> DDPIRPPLKVARSPRPGQCQDVVQDVPNVDVQMLELYDRMSFKDIDGGVWKQGWNIKYDPLKYNAHHKLKVFVVPHSHNDPGWIQTFEEYYQHDTKHILSNALRHLHDNPEMKFIWAEISYFARFYHDLGENKKLQMKSIVKNGQLEFVTGGWVMPDEANSHWRNVLLQLTEGQTWLKQFMNVTPTASWAIDPFGHSPTMPYILQKSGFKNMLIQRTHYSVKKELAQQRQLEFLWRQIWDNKGDTALFTHMMPFYSYDIPHTCGPDPKVCCQFDFKRMGSFGLSCPWKVPPRTISDQNVAARSDLLVDQWKKKAELYRTNVLLIPLGDDFRFKQNTEWDVQRVNYERLFEHINSQAHFNVQAQFGTLQEYFDAVHQAERAGQAEFPTLSGDFFTYADRSDNYWSGYYTSRPYHKRMDRVLMHYVRAAEMLSAWHSWDGMARIEERLEQARRELSLFQHHDGITGTAKTHVVVDYEQRMQEALKACQMVMQQSVYRLLTKPSIYSPDFSFSYFTLDDSRWPGSGVEDSRTTIILGEDILPSKHVVMHNTLPHWREQLVDFYVSSPFVSVTDLANNPVEAQVSPVWSWHHDTLTKTIHPQGSTTKYRIIFKARVPPMGLATYVLTISDSKPEHTSYASNLLLRKNPTSLPLGQYPEDVKFGDPREISLRVGNGPTLAFSEQGLLKSIQLTQDSPHVPVHFKFLKYGVRSHGDRSGAYLFLPNGPASPVELGQPVVLVTKGKLESSVSVGLPSVVHQTIMRGGAPEIRNLVDIGSLDNTEIVMRLETHIDSGDIFYTDLNGLQFIKRRRLDKLPLQANYYPIPSGMFIEDANTRLTLLTGQPLGGSSLASG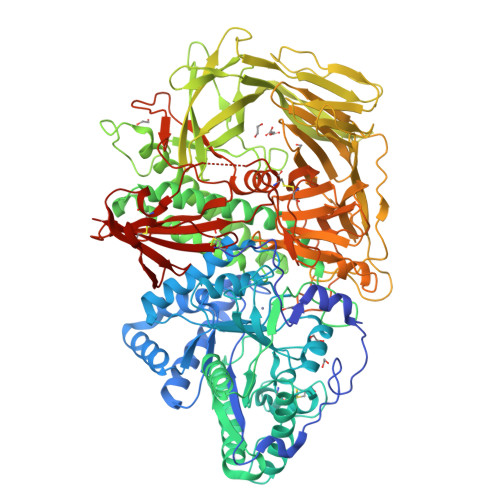ELEIMQDRRLASDDERGLGQGVLDNKPVLHIYRLVLEKVNNCVRPSELHPAGYLTSAAHKASQSLLDPLDKFIFAENEWIGAQGQFGGDHPSAREDLDVSVMRRLTKSSAKTQRVGYVLHRTNLMQCGTPEEHTQKLDVCHLLPNVARCERTTLTFLQNLEHLDGMVAPEVCPMETAAYVSSHSS>[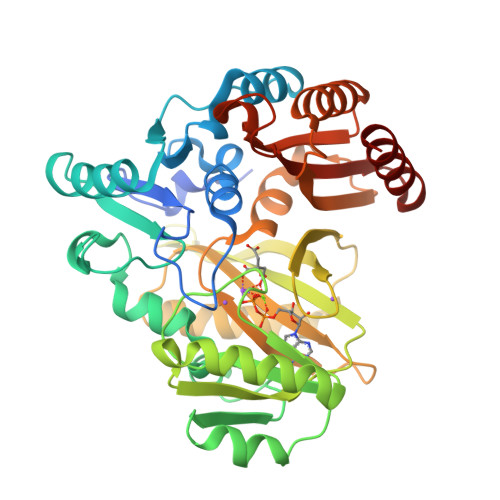2x]MHHHHHHHHMTNNGNEPNLTLSDLYDKDVVYTSRPSYISNPWLKPDEHQSNFLTGRELLIANQLPVIVHEASATDKLHQLFQVIGKEVPNSIYTFNNQQSYENLIKQLAHKENKKIYFQYIHDETILNQQYYALDKTLFVALNNKARIPEWTNGKFLPKRKVVKIEQFENEIKNWEFPLVIKPGDDLPTAGGYGVMICYHDADLQKAITRIKEATAETNSLIIEQKIEEKANYCVQFAYSESLGIQYLGAATQLTDKYGFYNGNENTTNVPEHVIEAGRQIMENGVNQGFFGVAGFDLLVDEDDNVYAIDLNFRQNGSTSMLLLANELNSGYQKFYSYHSKGDNTHFFNTILKYVKEGSLYPLSYYDGDWYGEDKVKSRFGCIWHGDSKETVLENERAFLAELEHY> MSAYATQGFNLDDRGRRIVVDPVTRIEGHMRCEVNVDANNVIRNAVSTGTMWRGLEVILKGRDPRDAWAFVERICGVCTGCHALASVRAVENALDIRIPKNAHLIREIMAKTLQVHDHAVHFYHLHALDWVDVMSALKADPKRTSELQQLVSPAHPLSSAGYFRDIQNRLKRFVESGQLGPFMNGYWGSKAYVLPPEANLMAVTHYLEALDLQKEWVKIHTIFGGKNPHPNYLVGGVPCAINLDGIGAASAPVNMERLSFVKARIDEIIEFNKNVYVPDVLAIGTLYKQAGWLYGGGLAATNVLDYGEYPNVAYNKSTDQLPGGAILNGNWDEVFPVDPRDSQQVQEFVSHSWYKYADESVGLHPWDGVTEPNYVLGANTKGTRTRIEQIDESAKYSWIKSPRWRGHAMEVGPLSRYILAYAHARSGNKYAERPKEQLEYSAQMINSAIPKALGLPETQYTLKQLLPSTIGRTLARALESQYCGEMMHSDWHDLVANIRAGDTATANVDKWDPATWPLQAKGVGTVAAPRGALGHWIRIKDGRIENYQCVVPTTWNGSPRDYKGQIGAFEASLMNTPMVNPEQPVEILRTLHSFDPCLACSTH;> METKPRTPVLWLHGLECTCCSESFIRSAHPLAKDVVLSMISLDYDDTLMAAAGHQAEAILEEIMTKYKGNYILAVEGNPPLNQDGMSCIIGGRPFIEQLKYVAKDAKAIISWGSCASWGCVQAAKPNPTQATPVHKVITDK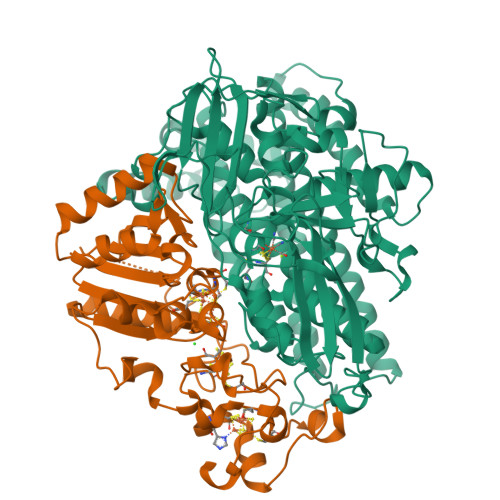PIIKVPGCPPIAEVMTGVITYMLTFDRIPELDRQGRPKMFYSQRIHDKCYRRPHFDAGQFVEEWDDESARKGFCLYKMGCKGPTTYNACSTTRWNEGTSFPIQSGHGCIGCSEDGFWDKGSFYDRLTGISQFGVEANADKIGGTASVVVGAAVTAHAAASAIKRASKKNETSGSEHRSAWSHPQFEK> MNILLFGKTGQVGWELQRSLAPVGNLIALDVHSKEFCGDFSNPKGVAETVRKLRPDVIVNAAAHTAVDKAESEPELAQLLNATSVE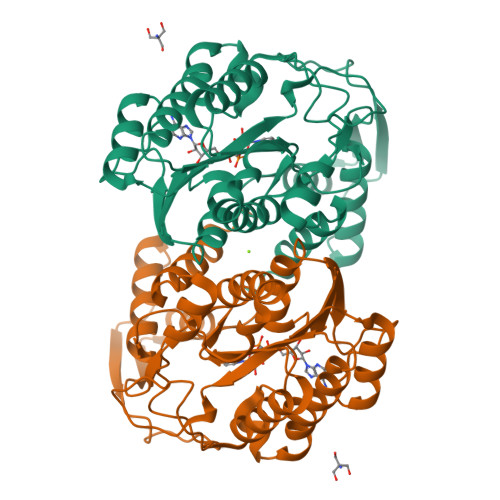AIAKAANETGAWVVHYSTDYVFPGTGDIPWQETDATSPLNVYGKTKLAGEKALQDNCPKHLIFRTSWVYAGKGNNFAKTMLRLAKERQTLSVINDQYGAPTGAELLADCTAHAIRVALNKPEVAGLYHLVAGGTTTWHDYAALVFDEARKAGITLALTELNAVPTSAYPTPASRPGNSRLNTEKFQRNFDLILPQWELGVKRMLTEMFTTTTI>MAFSVNYDSSFGGYSIHDYLGQWASTFGDVNHTNGNVTDANSGGFYGGSLSGSQYAISSTANQVTAFVAGGNLTYTLFNEPAHTLYGQLDSLSFGDGLSGGDTSPYSIQVPDVSFGGLNLSSLQAQGHDGVVHQVVYGLMSGDTGALETALNGILDDYGLSVNSTFDQVAAATAVGVQHADSPELLAA[2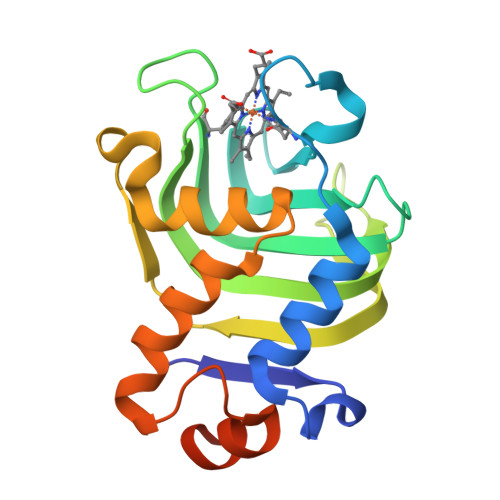x]>AECSVDIQGNDQMQFNTNAITVDKSCKQFTVNLSHPGNLPKNVMGHNMVLSTAADMQGVVTDGMASGLDKDYLKPDDSRVIAHTKLIGSGEKDSVTFDVSKLKEGEQYMF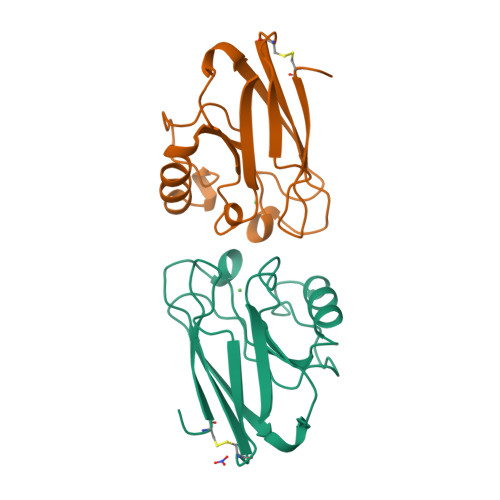FCTFPGHSALMKGTLTLK[4x]>SDTLPVSTCPAGQKYDRSVCYKADKIRSFCVANPRSNREKITDTPCQPREICVQRNLSNGKSFAKCIPIVDLVEWKTSANGNKEGCTTTSVNPAGYHHLGTIVYDINKNPIEVDKISYFGEPGNVNEGIGGSTSYFSSDNFQFSKSRYMKTCIFSGGYGNLNAYTWSWES[2x];> GPMGPLAQTESESADVAEHTINYIDIAPEEFEPPKANLSSLVENLYFQ

Plant pathogens secrete proteins, known as effectors, that function in the apoplast or inside plant cells to promote virulence. Previous studies of Fol-infected tomato identified a number of fungal proteins within the xylem sap. These secreted in xylem (SIX) effector proteins represent major pathogenicity determinants across different formae speciales of F. oxysporum. Currently, 14 SIX effectors have been identified in Fol consisting of small (less than 300 amino acids in length), secreted, cysteine-rich proteins. Here, we demonstrate that despite their sequence diversity, the Fol SIX effectors can be classified into a reduced set of structural families.

We analysed the cysteine spacing of the other SIX effectors and found that SIX6 and SIX13 contained a cysteine profile like Avr1 and Avr3, suggesting that they may be FOLD effectors. We subsequently generated SIX6 and SIX13 models, downstream of the predicted Kex2 cleavage site (SIX658-225, SIX1378-293), using AlphaFold2 and obtained high average confidence scored models supporting their inclusion in the FOLD family. To validate this experimentally, we produced SIX658-225 and SIX1322-293 (hereafter referred to as SIX6 and SIX13) as described for Avr1/Avr3 and obtained crystals for both proteins. While the SIX13 crystals diffracted poorly, the SIX6 crystals diffracted X-rays to ~1.9 Å, and we solved the structure of SIX6 using the AlphaFold2-generated model as a template for molecular replacement, confirming its inclusion as a member of the FOLD family. Despite lacking an N-terminal helix, the N-domain contains five β-strands held together by three disulfide bonds with an arrangement, identical to Avr1 and Avr3. The C-domain is an eight stranded β-sandwich that is stabilised by a single disulfide bond (unique to SIX6 compared to Avr1 and Avr3) connecting the β7 and β12 strands. Like Avr1, we identified regions of the pro-domain within the SIX6 structure (residues 29–46), despite cleavage of the pro-domain prior to crystallisation, but only within one molecule in the asymmetric unit. For structural analysis, we used the structured region of Chain A of SIX6. Despite this, AlphaFold2 models were critical in solving the structure of SIX6 and SIX8 as templates for molecular replacement. This negated the need to derivatise our crystals, a process that we had struggled with for SIX6 crystals, significantly reducing the time and research effort to determine the experimental structures.4-azanyl-6-[1-[[3,4-bis(fluoranyl)phenyl]methyl]pyrazol-4-yl]pyrimidine-5-carbonitrile | C15 H10 F2 N6 | 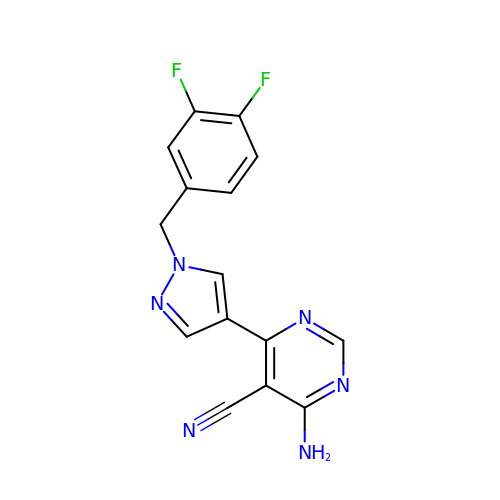XIBXZPKIDAMNCF-UHFFFAOYSA-N> MAVRLTFDGQKLTWPGIGIFKATTGLPDLQWPDKQCVPDAAIPEGNYKLFIQFQGEAPIRNAADCDLGPSWGWSTIPRGQAAGTCEIYWANWGYNRIRLESADEKTRKACGGKRGGFYIHDSTKGYSHGCIEVEPVFFRILKQETEKENGEKTF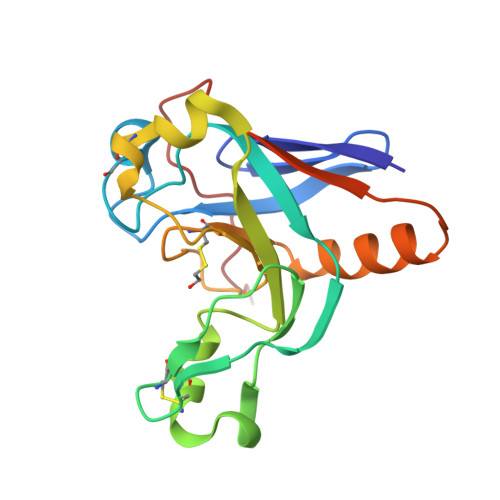TVNVKYVSGQQTNGGTKQGE> MKSSHHHHHHENLYFQSNAKQALLWRDSETFILTSIELYNWGGFQGYHRAEIDPSGTAVIGPTGSGKTTLVDALMTLLCANPRYNLASTGGHESDRDLVSYVRGVTGPGDGGVEQSHIARQGKTVTAIAATLERDGAQVRLGAVLWFEGTSSSASDLKKLWLLSESPEQTLEHWLSQHHAGGMRALRQMEKDGMGIWPYPSKKAFLARLRDYFEVGENAFTLLNRAAGLKQLNSIDEIFRELVLDDRSAFERAAEVASSF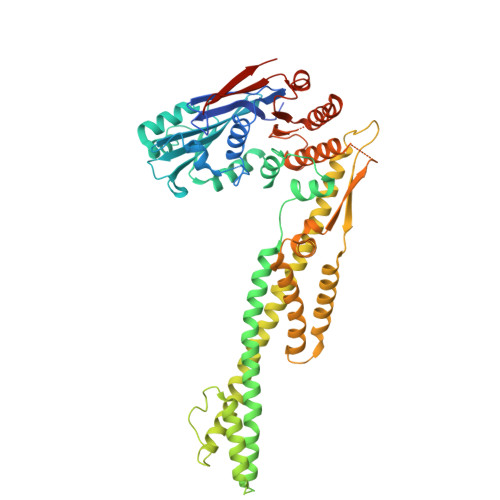DDLTDIHRELETARKQQRSLQPVADGWERYRALQEQLQDKQASGSSGSSGSSGQAKTLGEKLGDQKTELAKRMSDALKADTGALAEVGRELVDVPRYLERLRVLTEEALPEKLKRFLEYLNRSSDDGVTQLLSYIDHEVSMIEERLDDLNSTMQRVDFQPGRYLRLVAKKVIHESLRTLQHAQRQLNSARFIDDEGESHYKALQALVGLLKDACEHSRNQGAKALLDPRFRLEFAVSVIDREGNNLIETRTGSQGGSGGEKEIIASYVLTASLSYALCPDGSSRPLFGTIVLDQAFSRSSHAVAGRIIAALREFGLHAVFITPNKEMRLLRHHTRSAVVVHRRGVESSLVSLSWEALDEHHQQRIRAMHEVAH> ASQDQ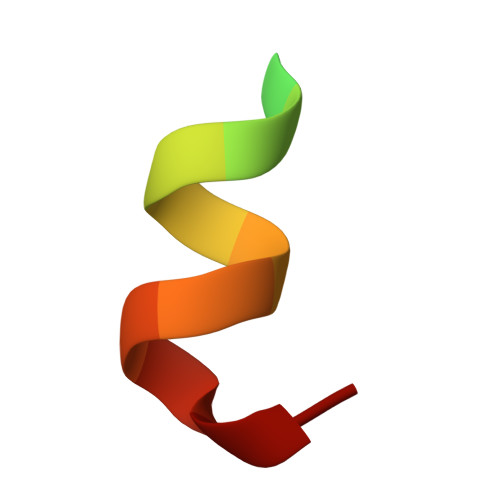VDDLLDSLGF> MSLINSRLAVAIHILSLISMDEKTSSEIIADSVNTNPVVVRRMISLLKKADILTSRAGVPGASLKKDPADISLLEVYRAVQKQEELFAVHENPNPKCPVG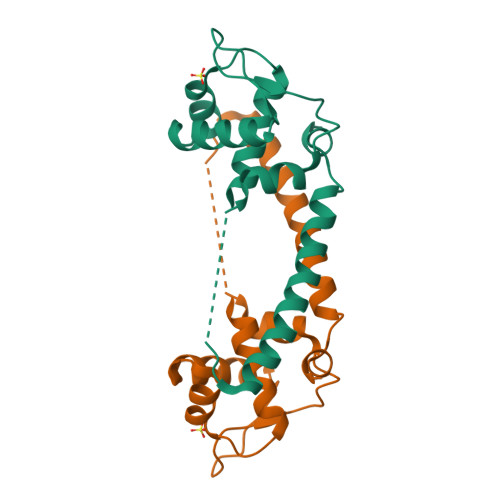KKIQNALDETFESVQRAMENELASKSLKDVMNHLFEGGSHHHHHH>[6x]MPKRGKKGAVAEDGDELRTEPEAKKSKTAAKKNDKEAAGEGPALYEDPPDQKTSPSGKPATLKICSWNVDGLRAWIKKKGLDWVKEEAPDILCLQETKCSENKLPAELQELPGLSHQYWSAPSDKEGYSGVGLLSRQCPLKVSYGIGDEEHDQEGRVIVAEFDSFVLVTAYVPNAGRGLVR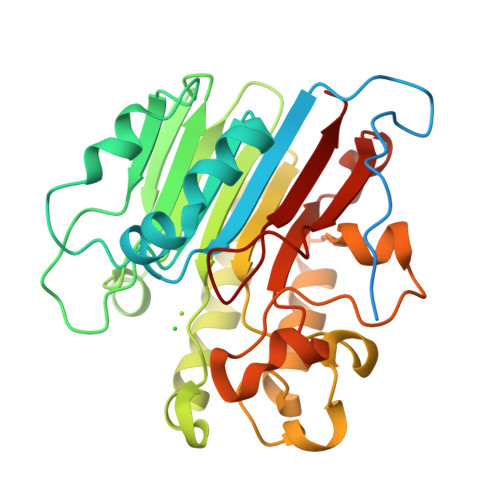LEYRQRWDEAFRKFLKGLASRKPLVLCGDLNVAHEEIDLRNPKGNKKNAGFTPQERQGFGELLQAVPLADSFRHLYPNTPYAYTFWTYMMNARSKNVGWRLDYFLLSHSLLPALCDSKIRSKALGSDHCPITLYLAL>AQVINTFDGVADYAQTYHKLPDNYITKSEAQALGWVASKGNLADVAPGKSIGGDIFSNREGKLPGKSGRTWREADINYT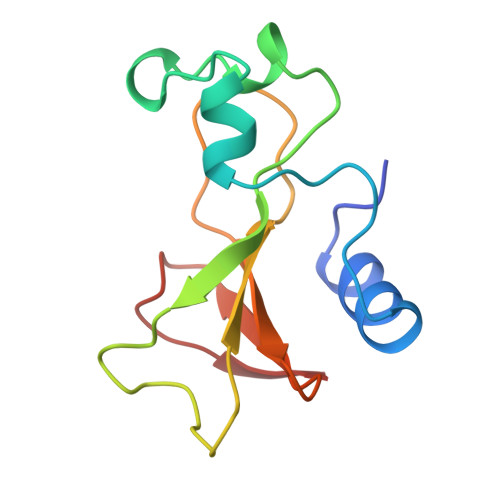SGFRNSDRILYSSDWLIYKTTDHYQTFTKIR[3x]> GSAGSGTIDDDDKSPGARGSMAEAGEILIKGGKVVNEDCSFFSDVHIRGGKIVEVGPDLRVPPGARVIDATDRLVIPGGIDTHTHMELAFMGTRAVDDFHIGTKAALAGGTTMILDFVMTQKGQSLLEAYDLWRKTADPKVCCDYSLHVAVTWWSDEVKDEMRTLAQERGVNSFKMFMAYKGLFMLRDDELYAVFSHCKEVGAIAQVHAENGDLIAEGAKKMLSLGITGPEGHELCRPEAVEAEATQRAITIASAVNCPLYV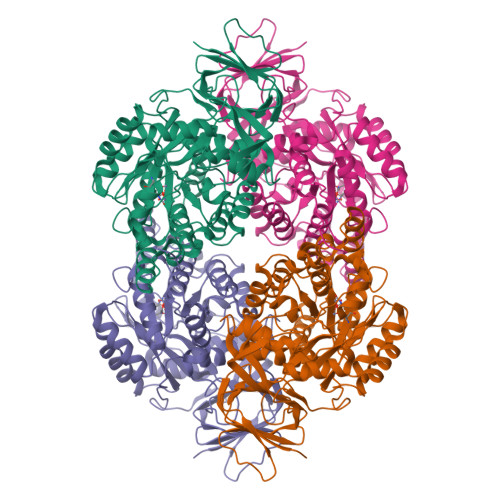VHVMSKSAADVVSKARKDGRVVFGEPIAASLGTDGTNYWHKDWAHAAQYVMGPPLRPDPSTPGYLMDLLANDDLTLTGTDNCTFSRCQKALGKDDFTRIPNGVNGVEDRMSVIWEKGVHSGKMDENRFVAVTSSNAAKIFNFYPQKGRIAKDSDADVVIWDPKTTRKISAQTHHQAVDYNIFEGMECHGVPVVTVSRGRVVYEEGRLKVSPGQGRFIHRQPFSEFVYKRIRQRDEVGKPAVVIREPYAGEVVALGTSD> QEDERIVLVDNKCKCARITSRIIRSSEDPNEDIVERNIRIIVPLNNRENISDPTSPLRTRFVY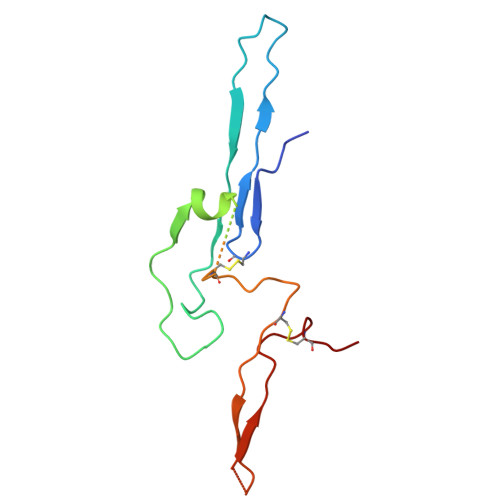HLSDLCKKCDPTEVELDNQIVTATQSNICDEDSATETCYTYDRNKCYTAVVPLVYGGETKMVETALTPDACYPD>MAKDKEFQVLFVLTILTLISGTIFYSTVEGLRPIDALFFSVVTLTTVGYGDFSPQTDFGKIFTI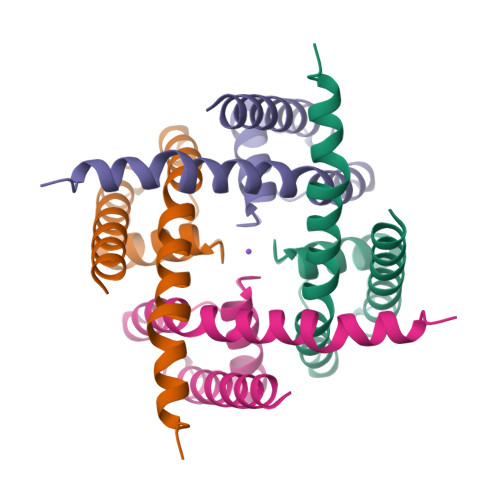LYIFIGIGLVFGFIHKLAVNVQLPSILSNLVPR[2x]> VEGAVKTEPVDLFHPGFLNSSNYRIPALFKTKEGTLIASIDARRHGGADAPNNDIDTAVRRSEDGGKTWDEGQIIMDYPDKSSVIDTTLIQDDETGRIFLLVTHFPSKYGFWNAGLGSGFKNIDGKEYLCLYDSSGKEFTVRENVVYDKDSNKTEYTTNALGDLFKNGTKIDNINSSTAPLKAKGTSYINLVYSD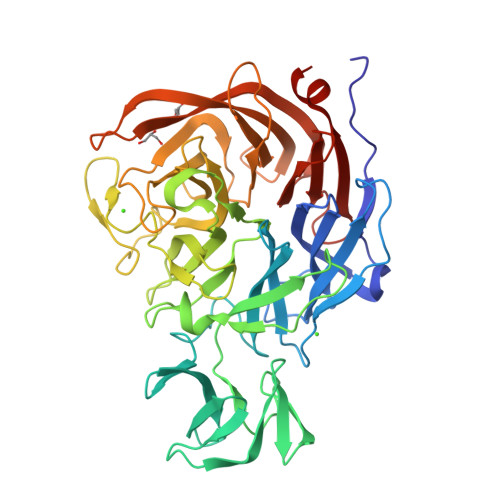DDGKTWSEPQNINFQVKKDWMKFLGIAPGRGIQIKNGEHKGRIVVPVYYTNEKGKQSSAVIYSDDSGKNWTIGESPNDNRKLENGKIINSKTLSDDAPQLTECQVVEMPNGQLKLFMRNLSGYLNIATSFDGGATWDETVEKDTNVLEPYCQLSVINYSQKVDGKDAVIFSNPNARSRSNGTVRIGLINQVGTYENGEPKYEFDWKYNKLVKPGYYAYSCLTELSNGNIGLLYEGTPSEEMSYIEMNLKYLESGANK> MAEVISISNATRVHSYRGVLIITDKLSVEAGSRASLSGYISDGGTSDVFTICRLLDAPMSGKPFISGNCSE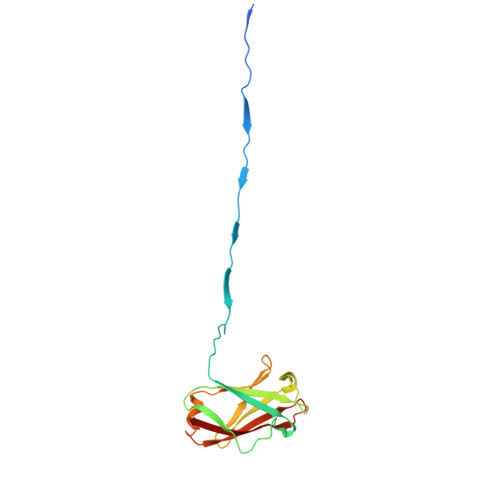IVKIPFDSSCLLGVKLYNCENKRINVNSIEAAFITLDTAFQSPMTVNKDTNRLEYIFSQNDYKVLVKGKVYDMIVNVVDESGNHSTVLKQKVRFN>[4x]MGLSLPKEKGLILCLWSKFCRWFQRRESWAQSRDEQNLLQQKRIWESPLLLAAKDNDVQALNKLLKYEDCKVHQRGAMGETALHIAALYDNLEAAMVLMEAAPELVFEPMTSELYEGQTALHIAVVNQNMNLVRALLARRASVSARATGTAFRRSPCNLI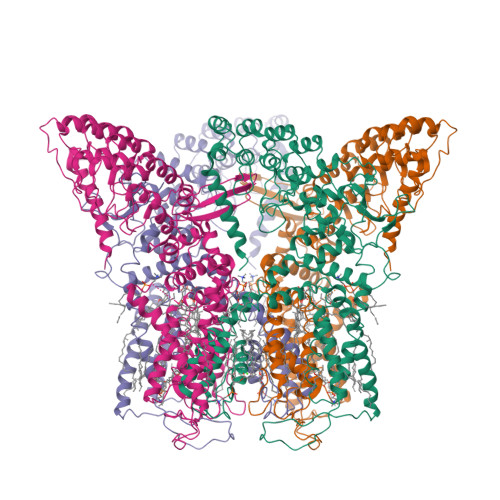YFGEHPLSFAACVNSEEIVRLLIEHGADIRAQDSLGNTVLHILILQPNKTFACQMYNLLLSYDRHGDHLQPLDLVPNHQGLTPFKLAGVEGNTVMFQHLMQKRKHTQWTYGPLTSTLYDLTEIDSSGDEQSLLELIITTKKREARQILDQTPVKELVSLKWKRYGRPYFCMLGAIYLLYIICFTMCCIYRPLKPRTNNRTSPRDNTLLQQKLLQEAYMTPKDDIRLVGELVTVIGAIIILLVEVPDIFRMGVTRFFGQTILGGPFHVLIITYAFMVLVTMVMRLISASGEVVPMSFALVLGWCNVMYFARGFQMLGPFTIMIQKMIFGDLMRFCWLMAVVILGFASAFYIIFQTEDPEELGHFYDYPMALFSTFELFLTIIDGPANYNVDLPFMYSITYAAFAIIATLLMLNLLIAMMGDTHWRVAHERDELWRAQIVATTVMLERKLPRCLWPRSGICGREYGLGDRWFLRVEDRQDLNRQRIQRYAQAFHTRGSEDLDKDSVEKLVPR> PMIIRGIRGARINNEIFNLGLK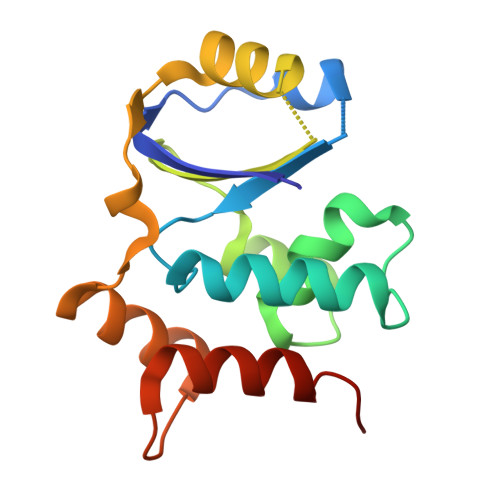FQILNADVVATKKHVLHAINQAKTKKPIAKSFWMEILVRASGQRQIHEAIKIIGAKDGNVCLICEDEETFRKIYELIGGEIDDSVLEINEDKERLIREIFKIRGFGNVVERVLEKIALIELKKE>GAMKVEVITGEEAESNVLQMQCKLFVFDKTSQSWVAVGRGLLRLNDMASTDDGTLQSRLVMRTQGSLRLILNTKLWAQMQIDKASEKSIRITAMDTEDQGVKVFLISASSKDTGQLYAALHHRILALRSRVEQEQEAK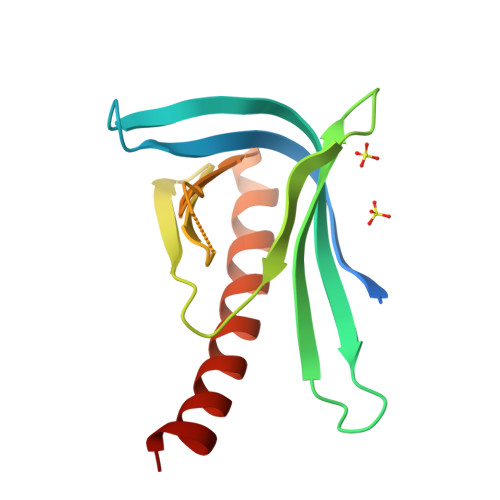[2x]>GSDFTWHRRYGHGVSEEDKGFGPIFEEQPINTIYPEESLEGKVSLNCRARASPFPVYKWRMNNGDVDLTNDRYSMVGGNLVINNPDKQKDAGVYYCLASNNYGMVRSTEATLSFGYLDPFPPEERPEVKVKEGKGMVLLCDPPYHFPDDLSYRWLLNEFPVFITMDKRRFVSQTNGNLYIANVESSDRGNYSCFVSSPSITKSVFSKFIPLIPIPERTTKPYPADIVVQFKDIYTMMGQNVTLECFALGNPVPDIRWRKVLEPMPSTAEISTSGAVLKIFNIQLEDEGLYECEAENIRGKDKHQARIYVQAFPEWVEHINDTEVDIGSDLYWPCIATGKPIPTIRWLKNGYSYHKGELRLYDVTFENAGMYQCIAENAYGSIYANAELKILALAPTFEMNPMKKKILAAKGGRVVIECKPKAAPKPKFSWSKGTEWLVNSSRILIWEDGSLEINNITRNDGGIYTCFAENNRGKANSTGTLVITNPTRIILAPINADITVGENATMQCAASFDPALDLTFVWSFNGYV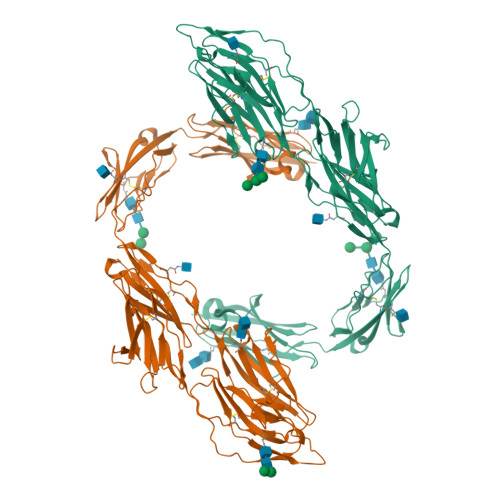IDFNKEITHIHYQRNFMLDANGELLIRNAQLKHAGRYTCTAQTIVDNSSASADLVVRGHHHHHH[2x]>[4x]MLVYNQEELVRFVEEAKQYARYGKVADYIPALGKANPNELSIAIYTPDDEVVSAGDVTVKVTLQSISKIIALALVLIDRGEDEVFHKVGMEPTDYPFHSIAK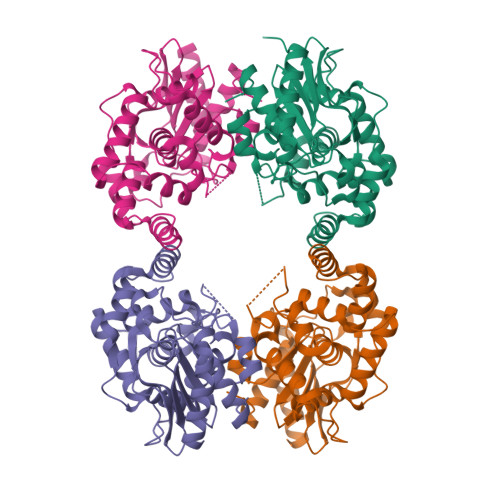LEEKPAKPLNPMINAGALVVTSMIQGGSVSERLERLLAFVRRLAGNERISYSDEVARSEFETAFLNRSLCYFLKQHRIIDEDVEELMELYTKQCAIEMTCIDLARIGLVLALDGRDPHSSEPLMPLDVARICKTFMVTCGMYNSSGEFAIKVGIPAKSGVSGGILAAVPGRCGIGVFGPALDDKGNSLTGVKLLERLSKTYSLSIF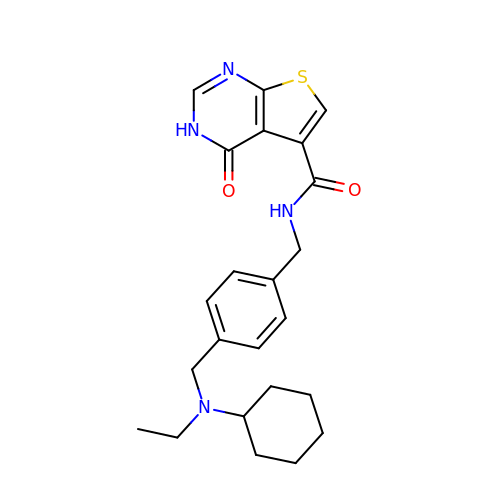N-[(4-{[cyclohexyl(ethyl)amino]methyl}phenyl)methyl]-4-oxo-3,4-dihydrothieno[2,3-d]pyrimidine-5-carboxamide | C23 H28 N4 O2 S | VDWQEXVBMIBDPI-UHFFFAOYSA-N> SGVIKPDMKIKLKMEGNVNGYAFVIEGEGEGKPYDGTNTINLEVKEGAPLPFSYDILTTAFAYGNRAFTKYPDDIPNYFKQSFPEGYSWERTMTFEDKGIVKVKSDISLEEDSFIYEIYLKGENFPPNGPVMQKKTTGWDASTERMYVRDGVLKGDVKHKLLLEGGGYYRVDFKTIYRAKKAVKLPDYHFVDHRIECLN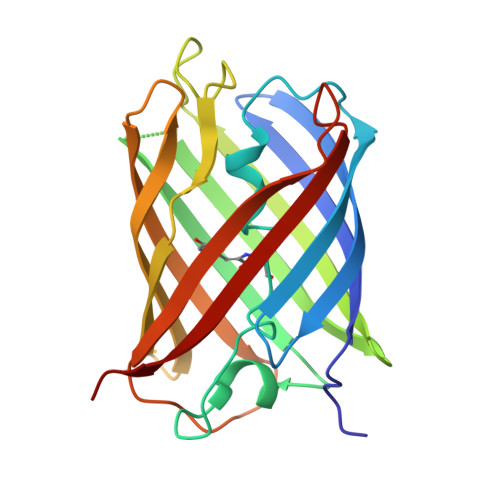HDKDHNKVTVYESAVARNSTD The curli biogenesis system in Enterobacteriaceae such as Salmonella species and Escherichia coli (E.coli), also known as the nucleation-precipitation or type VIII secretion system, is responsible for secreting curli subunits into the extracellular milieu to form cell associated nonbranching and highly aggregative amyloid fibrils. Lipoprotein CsgG forms a nonameric secretion channel in the outer membrane and transports CsgA and CsgB from periplasm into extracellular environment. Two soluble accessory factors, CsgE and CsgF, have been thought to bind to CsgG and play a crucial role in substrate (CsgA and CsgB) secretion and curli amyloid fiber formation. To address these questions, we determined the structures of complexes in curli biogenesis system by electron cryo-microscopy (cryoEM), including CsgF and CsgG (CsgFG) complexes both in the free for and bound to the N terminus (residues 1–22) of CsgA (CsgAN22).

The CsgFG complex structure was determined by single-particle cryo-EM at 3.8 Å resolution without any imposed symmetry. CsgG and CsgF were observed to bind together at a 9:9 stoichiometric ratio. By imposing C9 symmetry during three-dimensional (3D) reconstruction, the resolution was improved to 3.38 Å, which enabled unambiguous model building of entire CsgG subunit and N-terminal domain of CsgF (CsgFN, residues 1–36). In the 2D class averages, the CsgF C-terminal domain (CsgFC, residues 37–119) showed weak densities on the extracellular side of the channel, which reflected high flexibility of this domain in the complex. CsgFN was inserted into the CsgG channel β-barrel to form a layer inside the CsgG channel. Inside the CsgG channel, CsgFN was properly folded and contained a short α-helix. Each CsgFN subunit binds to two adjacent CsgG subunits mainly by hydrogen-bonds, electrostatic interactions, and hydrophobic interactions. In the presence of the CsgFG complex, we observed another pore structure formed by Asn17 of CsgFN, which was slightly larger (diameter of ~10.3 Å) than the one formed by CsgG (diameter of ~9 Å). Three phenylalanine mutations (F5D, F7D, and F12D) abolished the interaction between CsgF and CsgG. CsgFC was flexible, and was observed as fuzzy densities on the extracellular side of the CsgFG channel, which should be responsible for interacting with CsgB.

>[9x]MQRLFLLVAVMLLSGCLTAPPKEAARPTLMPRAQSYKDLTHLPAPTGKIFVSVYNIQDETGQFKPYPASNFSTAVPQSATAMLVTALKDSRWFIPLERQGLQNLLNERKIIRAAQENGTVAINNRIPLQSLTAANIMVEGSIIGYESNVKSGGVGARYFGIGADTQYQLDQIAVNLRVVNVSTGEILSSVNTSKTILSYEVQAGVFRFIDYQRLLEGEVGYTSNEPVMLCLMSAIETGVIFLINDGIDRGLWDLQNKAERQNDILVKYRHMSVPPES;>MRVKHAVVLLMLISPLSWAGTMTFQFRNPNFGGNPNNGAFLLNSAQAQNSYKDPSYNDDFGIETPSALDNFTQAIQSQILGGLLSNINTGKPGRMVTNDYIVDIANRDGQLQLNVTDRKTGQTSTIQVSGLQNNSTDF[9x]>MKIAIVGVSGAVGQEFLRVLSQRDFPIDGLYLFGSSRSAGSVYSFKGKEYVVRELKDNDDFKGIDIAFCSAGGDTSIAFADTITRHGTLMIDNSSAFRMQEDVPLVVPEVNGDDALVHPRNIISNPNCTTIQMVVALKPIEDLSHIRRVHVATYQAASGAGALGMAELVQQVEELARGEKPTVDKFAYQLMYNLIPQIDVFTDNDYTKEEMKMYRETKRIMHSDVMVSATCVRVPVMRAHSEAIWVETERPIAPEEARAAFAKAPGVLLCDEPSEKQYPMPLFGTEQDPVIVGRIRQDLANPN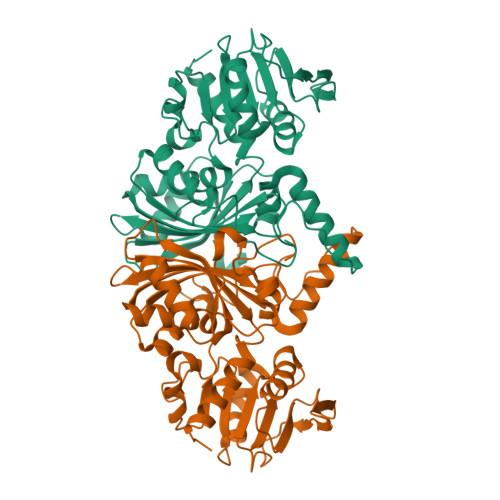GLVFWCVSDQIRKGAALNAVQIAEYLIAKGHFAR[2x]>[2x]MHHHHHHENLYFQGADQGSAEEVSVEELKAIQLRTTNEATGEKRFGSARA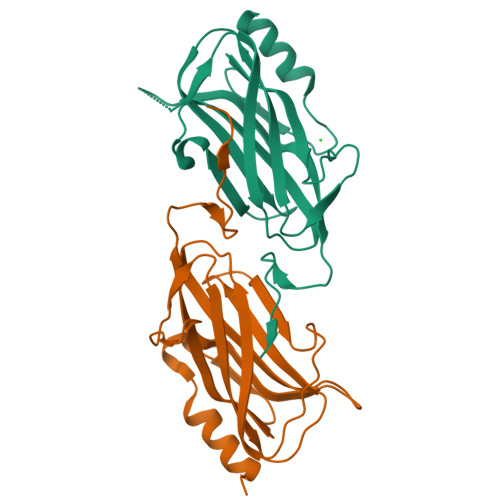IIEDLTIYKSDGTTLAEKPLIKSGEEVTFDFTILASEEIKDIALGISMSKAQGGDIWGDSNIGAGSAITLRPGRQRIVYKATLPINSGDYLIHCGLAKVGNGDREELDQRRPMMKVKFWSARELGGVIHAPLKIISNGES>[3x]KLKEIENRTRKPFEELCTELADLDMPAENIVLNRRVGQGAFGLVFGGEAKKSDLWEAVAVKVINEKANYEGKIDFLSEAKLMRSLNHPNVVRLIGISLNPKASLYLIMELMLLGDLKTYLLSRRILAQRSPNHEDIRPSTLTQMSMDIGQGLAYLHSKHLIHRDIACRNCLVAADRTVKIGDFGLTRQAAKNTSEAYYRFTRKCELPIRWMSPEAVQFGVFSIQSDIWSFGITLYEIITFGVFPYNGLGDVEVVERVKRMEFSITEFLPPQALNTVVCELINHCCKHQWQHRPSSMNQVLEVLIAYPDCIRPFLTDDPPKPNTTIDSLPFQPTVDTCIISE

Schistosoma mansoni Venus Kinase Receptors 1 and 2 (SmVKR1 and SmVKR2) are important for parasite growth and egg production, and are potential targets for combating schistosomiasis. VKRs consist of an extracellular Venus Flytrap Module (VFTM) linked via a transmembrane helix to a kinase domain. VKR proteins form homo- and heterodimers, a key requirement for VKR activation. The intracellular kinase domain of VKRs shares 41% sequence identity with that of insulin receptors (IRs).

To support our drug discovery approach, we determined for the first time a crystal structure of the SmVKR2KD at 3.0 Å resolution in the presence of ADP. SmVKR2 adopts a canonical bilobal kinase fold with an ADP molecule bound in the cleft between the two lobes. A novel feature of the SmVKR2KD is the presence of an extended helix at the N-terminal lobe, which we termed α0. This helix probably extends toward the membrane as part of the transmembrane helix that links the kinase domain with the VFTM module. The SmVKR2KD was crystallized as a dimer with the interface being stabilized by interactions between the N-lobe from one protomer and the C-lobe of the opposite protomer, related by a 2-fold symmetry. Although the crystals were grown in the presence of ATP-γ-S, the electron density maps only corresponded to the ADP moiety and not the thiophosphate group. As the crystals took over one month to grow, we believe that the ATP-γ-S was slowly hydrolyzed during crystallization and that we captured the posthydrolysis state of the kinase. Based on the conformation and orientation of the hydrophobic spine, the αC-in DFG-in conformation, and the E1014 and D1118 pointing toward the ATP-binding site, the SmVKR2KD has adopted an active-like conformation. In the SmVKR2KD, the loop is confined within the C-lobe reminiscent of active kinases, whereas in inactive kinases, it extends toward the N-lobe. Further, because the structure is in the presence of ADP, it most likely resembles the posthydrolysis state, and even though αC appears to be in the in-conformation, it shows a small degree of displacement toward the out-conformation relative to fully active kinases.>[2x]GPTYKYLQKPMYEVQWKVVEEINGNNYVYIDPTQLPYDHKWEFPRNRLSFGKTLGAGAFGKVVEATAYGLIKSDAAMTVAVKMLKPSAHLTEREALMSEL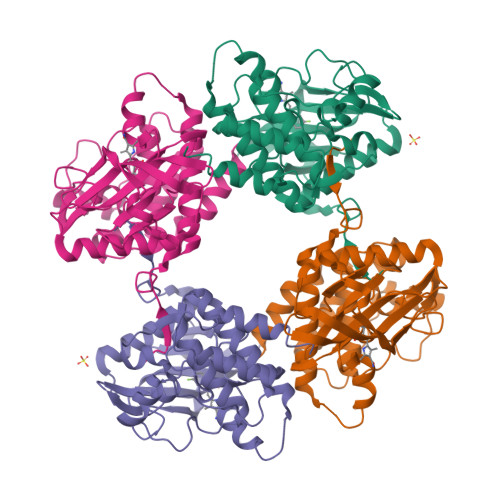KVLSYLGNHMNIVNLLGACTIGGPTLVITEYCCYGDLLNFLRRKRDSFICSKTSPAIMEDDELALDLEDLLSFSYQVAKGMAFLASKNCIHRDLAARNILLTHGRITKICDFGLARHIKNDSNYVVKGNARLPVKWMAPESIFNCVYTFESDVWSYGIFLWELFSLGSSPYPGMPVDSKFYKMIKEGFRMLSPEHAPAEMYDIMKTCWDADPLKRPTFKQIVQLIEKQISESTNHI[(2~{R},3~{S},4~{S},5~{R})-3,4-bis(oxidanyl)-5-[3-[4-[(~{E})-phenylcarbonyliminomethyl]-1,2,3-triazol-1-yl]propyl]oxan-2-yl]methyl 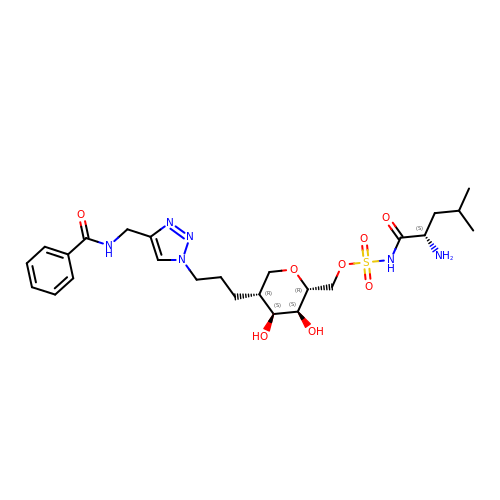~{N}-[(2~{S})-2-azanyl-4-methyl-pentanoyl]sulfamate | C25 H38 N6 O8 S | DTPWNCFCVLJKIS-ZADIZFFCSA-N> MSMAMSQSNRELVVDFLSYKLSQKGYSWSQFSDVEENRTEAPEGTESEAVKQALREAGDEFELRYRRAFSDLTSQLHITPGTAYQSFEQVVNELFRDGVNWGRIVAFFSFGGALCVES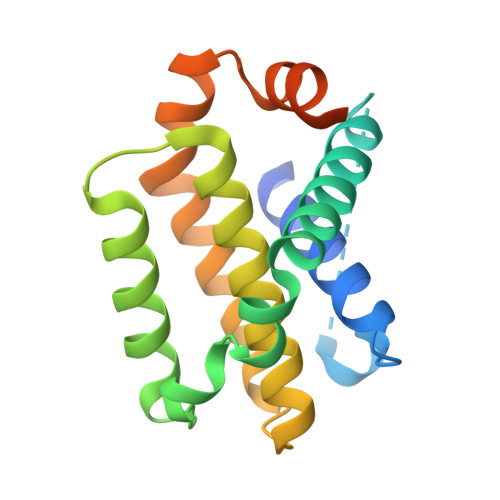VDKEMQVLVSRIAAWMATYLNDHLEPWIQENGGWDTFVELYGNNAAAESRKGQERLEHHHHHH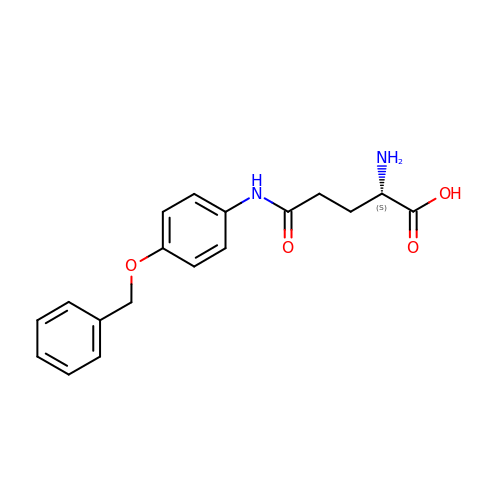(2S)-2-amino-5-oxo-5-[(4-phenylmethoxyphenyl)amino]pentanoic acid | C18 H20 N2 O4 | BYSBXIPCDJNEBG-INIZCTEOSA-N(2~{R},3~{S},4~{R},5~{R})-2-(aminomethyl)-5-[8-[3-[[(2~{R},3~{S},4~{R},5~{R})-5-(6-aminopurin-9-yl)-3,4-bis(oxidanyl)oxolan-2-yl]methoxy]prop-1-ynyl]-6-azanyl-purin-9-yl]oxolane-3,4-diol 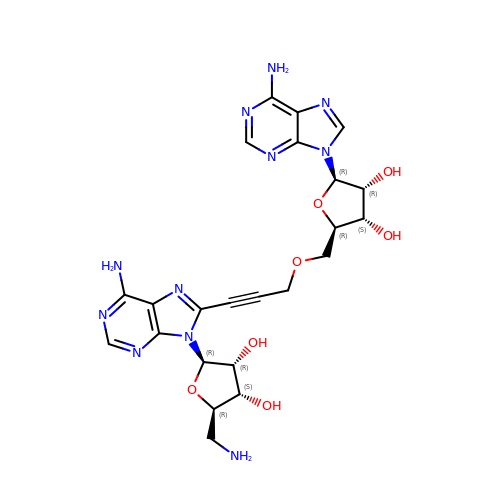| C23 H27 N11 O7 | NNTKMVAYMCZJCQ-MKWZPUSRSA-N>[2x]MGSITENTSWNKEFSAEAVNGVFVLCKSSSKSCATNDLARASKEYLPAATFKIPNAIIGLETGVIKNEHQVFKWDGKPRAMKQWERDLTL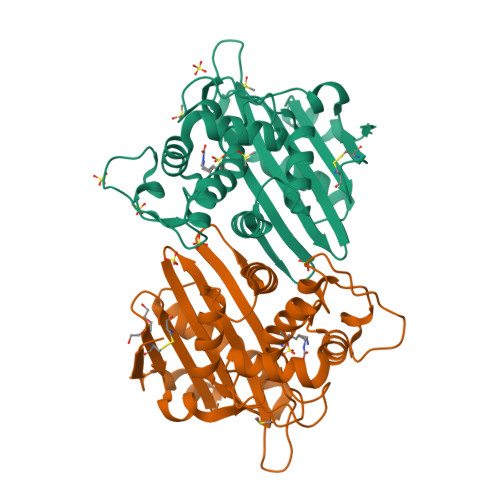RGAIQVSAVPVFQQIAREVGEVRMQKYLKKFSYGNQNISGGIDKFWLEGQLRISAVNQVEFLESLYLNKLSASKENQLIVKEALVTEAAPEYLVHSKTGFSGVGTESNPGVAWWVGWVEKETEVYFFAFNMDIDNESKLPLRKSIPTKIMESEGIIGG(11R,14S)-17-amino-14-hydroxy-8,14-dioxo-9,13,15-trioxa-14lambda~5~-phosphaheptadecan-11-yl decanoate | C23 H46 N O8 P | 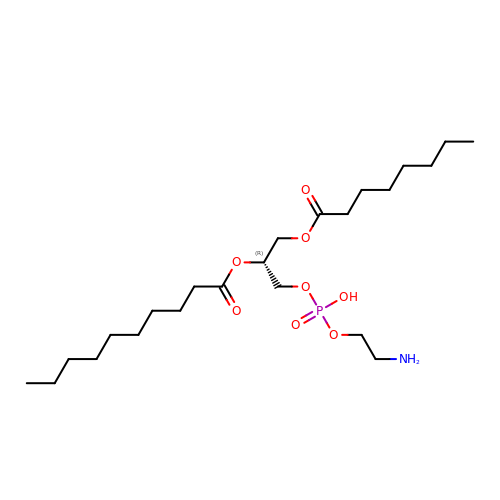VYUSSAVVRCGYLY-OAQYLSRUSA-N>[2x]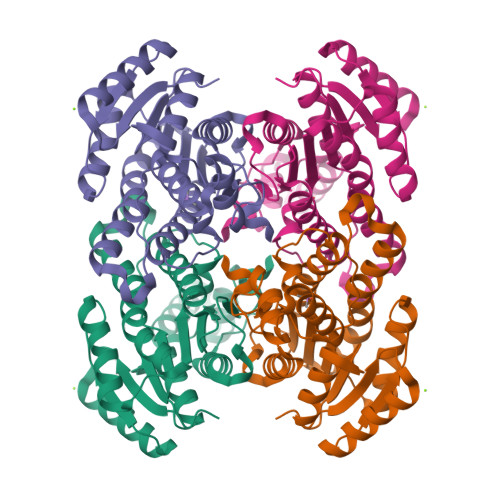MLKGKVAVVTGSTSGIGLGIATALAAQGADIVLNGFGDAAEIEKVRAGLAAQHGVKVLYDGADLSKGEAVRGLVDNAVRQMGRIDILVNNAGIQHTALIEDFPTEKWDAILALNLSAVFHGTAAALPHMKKQGFGRIINIASAHGLVASANKSAYVAAKHGVVGFTKVTALETAGQGITANAICPGWVRTPLVEKQISALAEKNGVDQETAARELLSEKQPSLQFVTPEQLGGTAVFLASDAAAQITGTTVSVDGGWTAR ERGIC-53 transports certain subsets of newly synthesized secretory proteins and membrane proteins from the endoplasmic reticulum to the Golgi apparatus. MCFD2 is a small protein composed of an EF-hand domain with two Ca2+ binding sites, and functions as a binding partner of ERGIC-53 in a Ca2+-dependent manner. From the amino acid sequence, ERGIC-53 is predicted to be a single-pass transmembrane protein that consists of a luminal carbohydrate recognition domain (CRD), a long stalk domain, a transmembrane (TM) helix and a short cytoplasmic tail (CT). Here we present cryo-EM structures of full-length ERGIC-53 in complex with its functional partner MCFD2. These structures reveal that ERGIC-53 exists as a homotetramer, not a homohexamer as previously suggested, and comprises a four-leaf clover-like head and a long stalk composed of three sets of four-helix coiled-coil followed by a transmembrane domain.

Consequently, we determined the cryo-EM structures of the head region of full-length ERGIC-53 complexed with MCFD2 in two forms (forms A and B) at 2.53 and 2.59 Å resolutions, respectively. Two different forms (A and B) of the head region are determined, in which the positions and orientations of the CRDs relative to the S-H2 are different. The superimposition on the central S-H2 coiled-coil demonstrates that during the conversion from form A to form B, the upper and lower CRDs rotate by 4.8˚ as a rigid body. Consequently, interface-H in form B is formed by interactions between different residues, such as van der Waals contact between Gln191 and Glu228’, while interface-V is almost maintained. These results suggest that interface-V involves tight binding, whereas interface-H is variable. As a result, the vertically assembled pair of CRDs can rotate to a certain extent (by 4.8˚) as a rigid body.

>[4x]MAGSRQRGLRARVRPLFCALLLSLGRFVRGDGVGGDPAVALPHRRFEYKYSFKGPHLVQSDGTVPFWAHAGNAIPSSDQIRVAPSLKSQRGSVWTKTKAAFENWEVEVTFRVTGRGRIGADGLAIWYAENQGLEGPVFGSADLWNGVGIFFDSFDNDGKKNNPAIVIIGNNGQIHYDHQNDGASQALASCQRDFRNKPYPVRAKITYYQNTLTVMINNGFTPDKNDYEFCAKVENMIIPAQGHFGISAATGGLADDHDVLSFLTFQLTEPGKEPPTPDKEISEKEKEKYQEEFEHFQQELDKKKEEFQKGHPDLQGQPAEEIFESVGDRELRQVFEGQNRIHLEIKQLNRQLDMILDEQRRYVSSLTEEISKRGAGMPGQHGQITQQELDTVVKTQHEILRQVNEMKNSMSETVRLVSGMQHPGSAGGVYETTQHFIDIKEHLHIVKRDIDNLVQRNMPSNEKPKCPELPPFPSCLSTVHFIIFVVVQTVLFIGYIMYRSQQEAAAKKFFGVAMPGAEDDVV;>GSHMEEPAASFSQPGSMGLDKNTVHDQEHIMEHLEGVINKPEAEMSPQELQLHYFKMHDYDGNNLLDGLELSTAITHVHKEEGSEQAPLMSEDELINIIDGVLRDDDKNNDGYIDYAEFAKSLQ[4x]>MLVKGNEILLKAHKEGYGVGAFNFVNFEMLNAIFEAGNEENSPLFIQASEGAIKYMGIDMAVGMVKIMCERYPHIPVALHLDHGTTFESCEKAVKAGFTSVMIDASHHAFEENLELTSKVVKMAHNAGVSVEAELGRLMGIEDNISVDEKDAVLVNPKEAEQFVKESQVDYLAPAIGTSHGAFKFKGEPKLDFERLQEVKRLTNIPLVLHGASAIPDNVRKSYLDAGGDLKGSKGVPFEFLQESVKGGINKVNTDTDLRIAFIAEVRKVANEDKSQFDLRKFFSPAQLALKNVVKERMK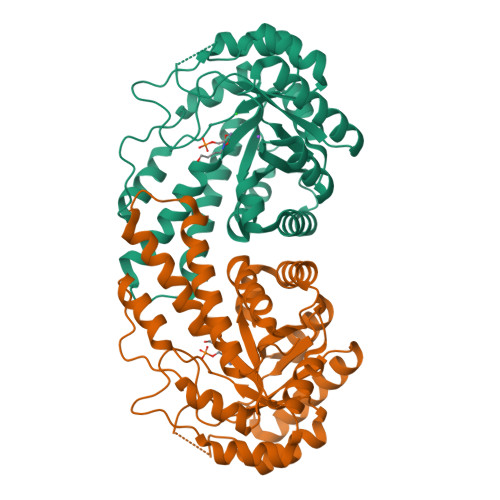LLGSANKI[8x]N-[3-({[(3S,5S)-5-{[(3-{[(Z)-imino(thiophen-2-yl)methyl]amino}benzyl)oxy]methyl}pyrrolidin-3-yl]oxy}methyl)phenyl]thiophene-2-carboximidamide 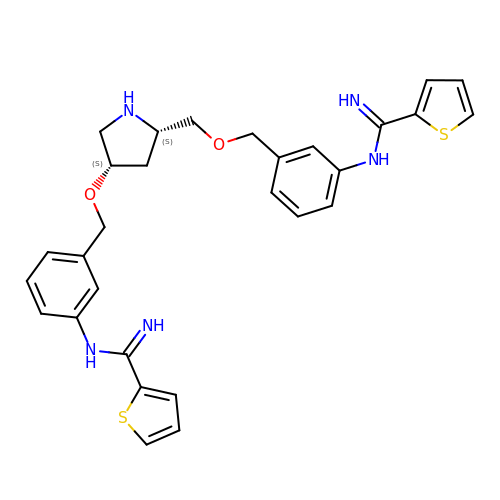| C29 H31 N5 O2 S2 | GPVRORSBZUBDJB-DQEYMECFSA-N6-methoxy-1,3-benzothiazole-2-carboxylic 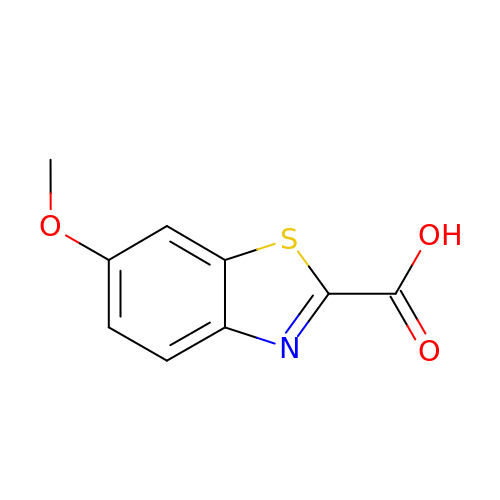acid | C9 H7 N O3 S | JDKMYJZEGZZJOH-UHFFFAOYSA-N> GRHVRSYNHLQGDVRWRKLFSFTKYFLKIEKNGKVSGTKKENCPYSILEITSVEIGVVAVKAINSNYYLAMNKKGKLYGSKEFNNDCKLKERIEENGYNTYASFNWQHNGRQMYVALNGKGAPRRGQKTRRKNTSAHFLPMVVHS;> AEDFVSENSNNKRAPYWTNTEKMEKRLHAVPAANTVKFRCPAGGNPMPTMRWLKNGKEFKQEHRIGGYKVRNQHWSLIMESVVPSDKGNYTCVVENEYGSINHTYHLDVVER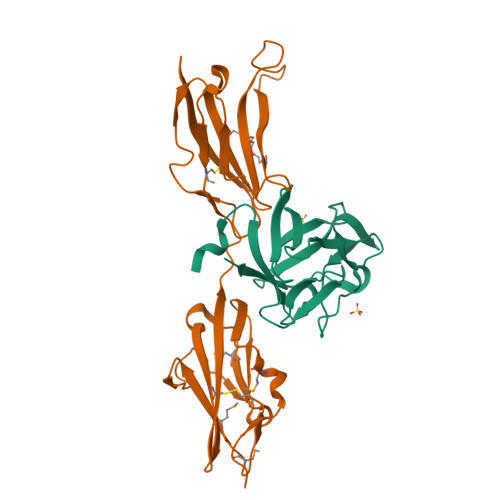SPHRPILQAGLPANASTVVGGDVEFVCKVYSDAQPHIQWIKHVEKNGSKYGPDGLPYLKVLKHSGINSSNAEVLALFNVTEADAGEYICKVSNYIGQANQSAWLTVLPKQQAPGREKE> MNINQLILRNLKKNLRNYYLYVFALIFSVALYFAFVTLQYDPAINEVKASIKGAAAIKTASILLVAVVAIFILYANTIFIKRRSKEIGLFQLIGMTKHKIFRILSAENVMLYFGSLAIGVAAGFSISKLVLMILFKIVDVKADAKLHFSEQALVQTVIVFCGIYLLIMIMNYTFIKKQSILSLFKVTSSTEDKVKKISFFQMLIGALGIVLILTGYYVSSELFGGKFKTINELFVAMSFILGSVIIGTFLFYKGSVTFISNIIRKSKGGYLNISEVLSLSSIMFRMKSNALLLTIITTVSALAIGLLSLAYISYYSSEKTAEQNVAADFSFMNEKDAKLFENKLRESNISFVKKATPVLQANVDIANIMDGTPKEMQGDPGNMQLAVVSDKDVKGVDVAAGEAVFSGYTDLLQKIMVFKDSGVIKVKSKHETQPLKYKGLREEFLVSYTFTSGGMPAVIVDDSLFKQLDKDKDPRIQLAQSTFIGVNVKHDDQMEKANELFQQVNKKNEHLSRLDTSAAQKSLFGMVMFIVGFLGLTFLITSGCILYFKQMGESEDEKPSYTILRKLGFTQGDLIKGIRIKQMYNFGIPLVVGLFHSYFAVQSGWFLFGSEVWAPMIMVMVLYTALYSIFGFLSVLYYKKVIKSSL;>MSGHHHHHHVILEANKIRKSYGNKLNKQEVLKGIDIHIEKGEFVSIMGASGSGKTTLLNVLSSIDQVSHGTIHINGNDMTAMKEKQLAEFRKQHLGFIFQDYNLLDTLTVKENILLPLSITKLSKKEANRKFEEVAKELGIYELRDKYPNEISGGQKQRTSAGRAFIHDPSIIFADEPTGALDSKSASDLLNKLSQLNQKRNATIIMVTHDPVAASYCGRVIFIKDGQMYTQLNKGGQDRQTFFQDIMKTQGVLGGVQHEH[2x];>[2x]MIKAFLIERRSWIAAFLFQQALMLFIAFVDPSISFGNVLYMVYLCILFFIIFLWFRYRKETAFYKSLKTWENNLDVTAINEPETPFEAMVERSIAGQTEHLKQTAARHRLALENEKDELMAWIHEVKTPLTAMHLIIDRMEEKALKSQLSYEWLRIHLLLDQQLHQKRISFIENDLSVEFIQLQPLIFKEIKDLQSWCIQKGIGFDIQLEAKEVLSDAKWLAFIIRQLLTNAVKYSEASEIEIKSFQKGEQTQLQVKDCGRGIDPKDVPRIFDKGFTSTTDHHDQASTGMGLYLAKKAAAPLLIHIDVESEFGAGTVFTLTFPIRNQFEHVISV

One such mechanism widely found across Firmicute bacteria involves antimicrobial peptide sensing and resistance membrane protein complexes collectively known as Bce modules. These modules are composed minimally of an ATP-binding cassette (ABC) transporter which defends against antimicrobial peptides without transport across the membrane, and an interacting two-component system containing a sensor histidine kinase and response regulator. In this module bceA encodes the ATPase domains, bceB encodes the membrane-spanning permease domain of the ABC transporter BceAB, and bceS encodes the histidine kinase that phosphorylates the response regulator encoded by bceR. Previous studies have established that BceAB mediates resistance against bacitracin, likely by freeing bacitracin from the lipid target undecaprenyl-pyrophosphate (UPP). To understand this critical membrane protein interaction and the molecular details underpinning the Bce module flux-sensing mechanism, we have determined the cryo-EM structure of the complete BceAB-S complex from B. subtilis in nucleotide-free and ATPγS-bound states.

Residual signal subtraction focused on the TM region was followed with a round of 3D classification without alignment, generating two distinct classes of particles with high-resolution features in the TM region. Refinement of these two classes independently produced separate 3D volumes each at ~3.4 Å overall resolution. We refer to these two reconstructions as TM-state-1 and TM-state-2. For simplicity we focus on TM state-1 for the following analysis. Within the detergent belt 14 total TM helices were clearly identified, with 10 belonging to BceB and another 4 belonging to the BceS dimer. The cryo-EM maps were of sufficient quality to build atomic models of TM1 and TM2 of each BceS monomer de novo. Several types of interactions mediate dimerization of two BceS monomers. In the middle of the bilayer plane is a cluster of aromatic residues including Trp12, Phe16, Phe49, and Phe52 that form an extensive π-stacking interaction network. The total buried surface area between BceB and the two BceS monomers is only ~460 Å2 near the apex of BceB-TM3, which contacts TM1 from one BceS monomer and TM2 from the second BceS monomer. Nevertheless, our cryo-EM structures clearly demonstrate that most of the interaction between BceB and BceS is mediated through protein-lipid interactions rather than direct protein–protein interaction.>[2x]NLVTAFSNMDDMLQKAHLVIEGTFI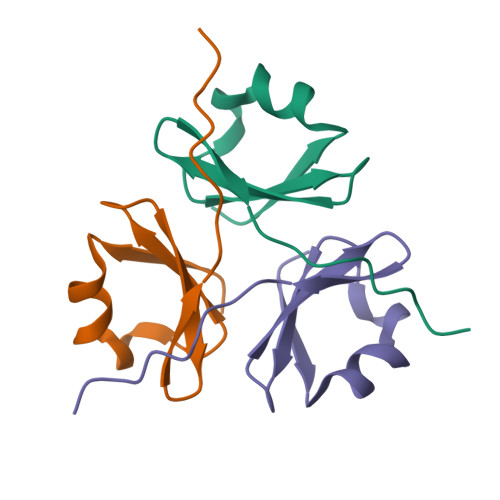YLRDSTEFFIRVRDGWKKLQLGELIPIPA>[2x]ANFMIYPISKDLKNGNSELVRVYSKSKEIQYIKIYTKKIINPGTTEEYEVDIPNWDGGLVVTPQKVILPAGASKSIRLTQFKIPKKEEVYRVYFEAVKPDSKENVIDNKKLTIEISINIIYAALIRSLPSEQNISLNISRNAKKNIIIYNNGNVRAGVKDIY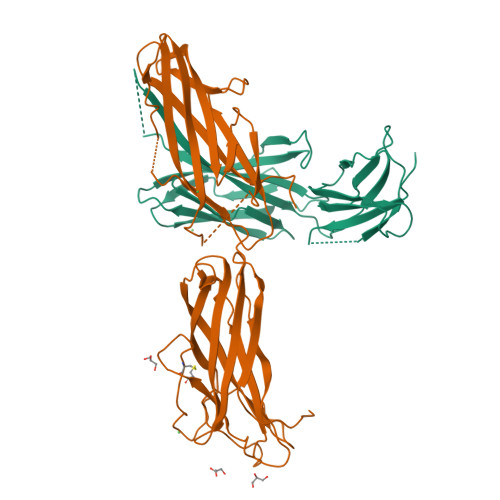FCKSSNIDDNCVKKAYNKNIYPEKSFDTLVNNNFSYVFIKLNHEGIEKEQGLIQLKVPA;>[2x]HHHHDKNPGSENMTNTIGPHDRGGSSPIYNILNSYLTAYNGSHHLYDRMSFLCLSSQNTLNGACPSSDAPGTATIDGETNITLQFTEKRSLIKRELQIKGYKQFLFKNANCPSKLALNSSHFQCNREQASGATLSLYIPAGELNKLPFGGVWNAVLKLNVKRRYDTTYGTYTINITVNLTDKGNIQIWLPQFKSNARVDLNLRPTGGGTYIGRNSVDMCFYDGYSTNSSSLEIRFQDDNSKSDGKFYLKKINDDSKELVYTLSLLLAGKNLTPTNGQALNINTASLETNWNRITAVTMPEISVPVLCWPGRLQLDAKVKNPEAGQYMGNIKITFTPSSQTL> SKKSGKSAKSKEKQEKITDTFKVKRKVDRFNGVSEAELLTKTLPDILTFNLDIVIIGIAPGLMAAYKGHHYPGPGNHFWKCLFMSGLS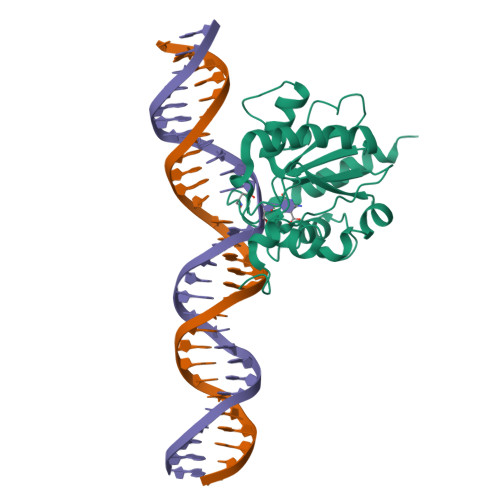EVQLNHMDDHTLPGKYGIGFTNMVERTTPGSKDLSSKEFREGGRILVQKLQKYQPRIAVFNGKCIYEIFSKEVFGVKVKNLEFGLQPHKIPDTETLCYVMPSSSARCAQFPRAQDKVHYYIKLKDLRDQLKGIERNMDV>[2x]MTGMSREEVESLIQEVLEVYPEKARKDRNKHLAVNDPAVTQSKKCIISNKKSQPGLMTIRGCAYAGSKGVVWGPIKDMIHISHGPVGCGQYSRAGRRNYYIGTTGVNAFVTMNFTSDFQEKDIVFGGDKKLAKLIDEVETLFPLNKGISVQSECPIGLIGDDIESVSKVKGAELSKTIVPVRCEGFRGVSQSLGHHIANDAVRDWVLGKRDEDTTFASTPYDVAIIGDYNIGGDAWSSRILLEEMGLRCVAQWSGDGSISEIELTPKVKLNLVHCYRSMNYISRHMEEKYGIPWMEYNFFGPTKTIESLRAIAAKFDESIQKKCEEVIAKYKPEWEAVVAKYRPRLEGKRVMLYIGGLRPRHVIGAYEDLGMEVVGTGYEFAHNDDYDRTMKEMGDSTLLYDDVTGYEFEEFVKRIKPDLIGSGIKEKFIFQKMGIPFREMHSWDYSGPYHGFDGFAIFARDMDMTLNNPCWKKLQAPWEASEGAEKVAASA;>MSQQVDKIKASYPLFLDQDYKDMLAKKRDGFEEKYPQDKIDEVFQWTTTKEYQELNFQREALTVNPAKACQPLGAVLCALGFEKTMPYVHGSQGCVAYYRSYFNRHFREPVSCVSDSMTEDAAVFGGQQNMKDGLQNCKATYKPDMIAVSTTCMAEVIGDDLNAFINNSKKEGFIPDEFPVPFAHTPSFVGSHVTGWDNMFEGIARYFTLKSMDDKVVGSNKKINIVPGFETYLGNFRVIKRMLSEMGVGYSLLSDPEEVLDTPADGQFRMYAGGTTQEEMKDAPNALNTVLLQPWHLEKTKKFVEGTWKHEVPKLNIPMGLDWTDEFLMKVSEISGQPIPASLTKERGRLVDMMTDSHTWLHGKRFALWGDPDFVMGLVKFLLELGCEPVHILCHNGNKRWKKAVDAILAASPYGKNATVYIGKDLWHLRSLVFTDKPDFMIGNSYGKFIQRDTLHKGKEFEVPLIRIGFPIFDRHHLHRSTTLGYEGAMQILTTLVN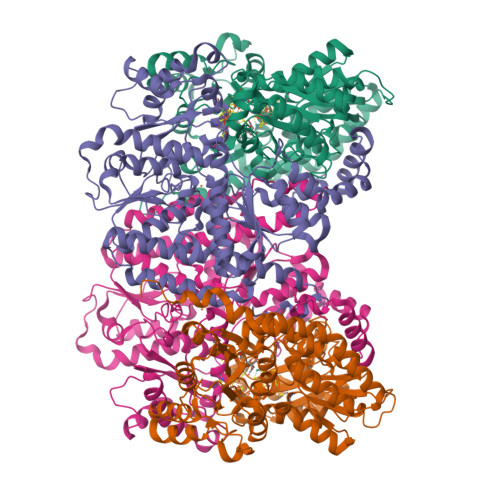SILERLDEETRGMQATDYNHDLVR[2x]> MINMARFDKKE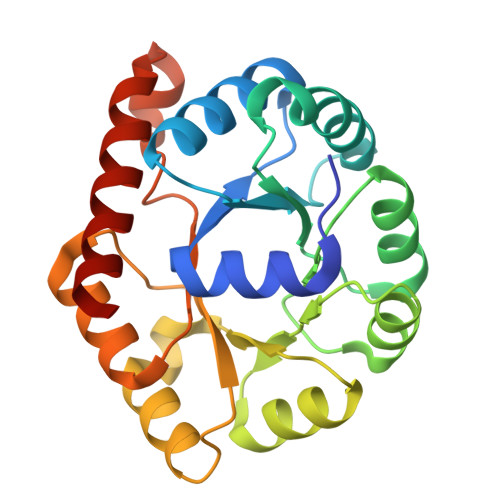TIRTMTDTGLVPVFCSCDVEVAKQVIRACYNGGVRVFEFTNREEAAHEVFGAVSRWIVEACPEMILGVGSIVDAPTASLYLQSGANFVVGPLTNPDIAKVCNRRLVPYIPGCGSVSEVGYAQELGCDICKVFPGDVLGPGFVKALKAPMPWSQVMVTGGVKPKEANLKAWFDAGATCVGMGSNLFPPEAIASGNWEKITDICAQALGVIREVRKE>GHMNQFVTNTKNVIRGKYHPEFLQNEVLADIFAHTAQTLPDKTALIEADKTLSYGELYQQALIMAQHLALKGVKPGHIVGLWLPRGIELLKAQLAICLSGAAWLPFDMDTPADRIAVCLEDAEAVGMITTDEWYEHLAEVPQTKWTNTELQKPLSESVSLAKTTPDQPAYIIYTSGSTGKPKGIVITQKNICHFLRSENSILGIQEQDKVYQGFSVAFDMSFEEIWLSYLVGATLWIAPKSLVSDPERLCQTLKQEQITVLHAVPTLLALFPEDVPNLRIINLGGEMCPDSLVDRWALPHHQMFNT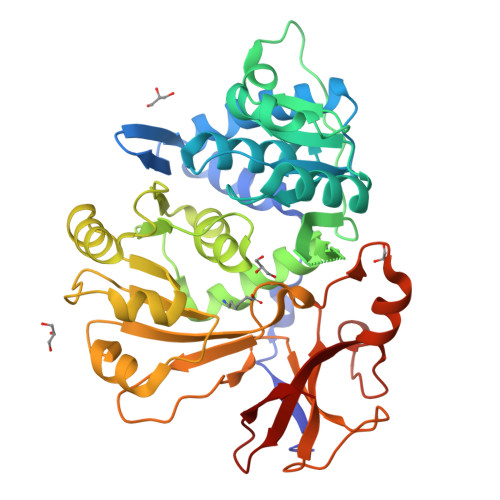YGPTETTVSASLELLERGKPVTIGKPLPNYGMLVINSERELLEQGETGELCIFGPSVAQGYLGRPDLTADKFIENPWAMSVEEELLYRTGDLAKIDEFGQVHCLGRA[2x]>MRGSHHHHHHGSMACPLEKALDVMVSTFHKYSGKEGDKFKLNKSELKELLTRELPSFLGKRTDEAAFQKLMS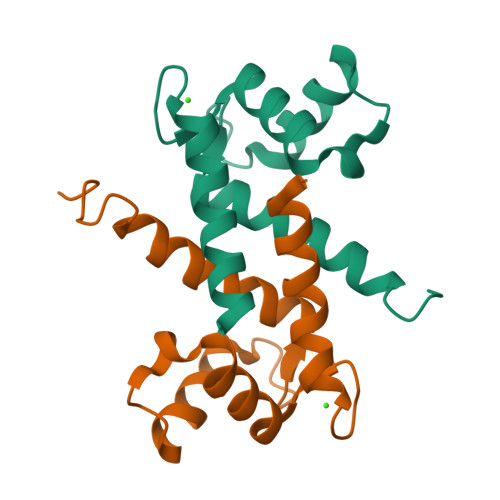NLDSNRDNEVDFQEYCVFLSCIAMMCNEFFEGFPDKQPRKK[4x]l-2-hydroxyglutarate dehydrogenase (L2HGDH) is a mitochondrial membrane–associated metabolic enzyme, which catalyzes the oxidation of l-2-hydroxyglutarate (l-2-HG) to 2-oxoglutarate (2-OG). L2HGDH belongs to the d-amino acid oxidase (DAAO) family of the FAD-dependent proteins. Like other members of the DAAO family, dmL2HGDH is composed of the FAD-binding domain and the substrate-binding domain. The active site of dmL2HGDH is located at the interface of the FAD-binding domain and the substrate-binding domain and is composed of residues from both domains.

Crystallization of dmL2HGDH in the absence of any ligands yielded crystals in FAD-bound form (dmL2HGDHFAD) and in complex with FAD and SO42− (dmL2HGDHFAD+SO4) in which SO42− was derived from the crystallization solution. Structures of dmL2HGDH in FAD-bound form and in complex with FAD and SO42− or 2-OG were determined at resolutions of 2.85 Å, 2.30 Å, and 2.82 Å, respectively. Structural comparison of dmL2HGDH in FAD-bound form and in complex with FAD and 2-OG shows that the 2-OG binding at the active site does not induce notable conformational changes of the residues involved in the FAD and ligand binding (RMSD of ∼0.37 Å for 412 aligned Cα atoms). In all structures, there are four dmL2HGDH monomers forming a tetramer in the asymmetric unit. The four monomers share almost identical conformation and are related by noncrystallographic 222 symmetry. In each monomer, there are an FAD bound at the active site and a detergent molecule n-dodecyl-β-d-maltopyranoside (DDM) on a surface groove. The FAD molecule is apparently derived from the expression system. In all structures, an FAD molecule is bound at the FAD-binding site, which adopts an elongated conformation with the isoalloxazine moiety pointing toward the substrate-binding site and forming extensive hydrophilic and hydrophobic interactions with the surrounding residues. On the si-face of the isoalloxazine moiety, the N5, O4, and N3 atoms form several hydrogen bonds with the main chains and side chains of Ser88 and Val90; on the re-face of the isoalloxazine moiety, the N3 atom forms hydrogen bonds with the side chain of His92. On the other hand, the A–B (or C–D) interface is mediated by both hydrophilic and hydrophobic interactions as well as a disulfide bond formed by two Cys77 residues.

>[4x]GDYDLVVVGGGIVGAASAREIVLRHPSLKVAVLEKECKLAKHQSGHNSGVIHAGIYYKPGTLKARLCVEGMHLAYAYLDEKKIPYKKTGKLIVATDEKEVKLLKDLEKRGIANNVPDLRMIEGSEIQEIEPYCQGVMALHSPHTGIVDWGLVTEHYGQDFKQCGGDIYLDFNVSKFTETKEGTDYPVTIHGAKPGQTVRTKNVLTCGGLQSDLLAEKTGCPRDPRIVPFRGEYLLLTKEKQHMVKGNIYPVPDPRFPFLGVHFTPRMDGSIWLGPNAVLALKREGYTWGDINLFELFDALRYPGFVKMASKYIGFGLSEMSKSWFINLQIKALQKYIPDITEYDIQRGPAGVRAQAMDLDGNLVDDFVFDRGQGSGALAKRVLHCRNAPSPGATSSLAIAKMIADKIENEFSIGK In response, one family of large bacteriophages uses a nucleus-like compartment to protect its replicating genomes by excluding host defence factors. Here we find that the bacteriophage nuclear shell assembles primarily from one protein, which we name chimallin (ChmA). Combining cryo-electron tomography of nuclear shells in bacteriophage-infected cells and cryo-electron microscopy of a minimal chimallin compartment in vitro, we show that chimallin self-assembles as a flexible sheet into closed micrometre-scale compartments. We find that the shell is primarily composed of a single protein, chimallin, which self-assembles through its extended N and C termini into a closed compartment.

Size-exclusion chromatography coupled to multi-angle light scattering (SEC–MALS) of purified chimallin indicated a mixture of oligomeric states including monomers, well-defined assemblies of approximately 1.2 MDa, and larger heterogeneous species ranging from 4 to 13 MDa (mean of 6.9 MDa). Cryo-ET of the largest species revealed pleomorphic, closed compartments with near-identical morphology to the phage nuclear shell that we observe in situ. Analysis of the smaller, more defined assemblies by cryo-ET revealed a near-homogeneous population of cubic assemblies with a diameter of around 22 nm, and a minor population of rectangular assemblies with dimensions of approximately 22 × 33.5 nm. Two-dimensional class averages revealed that each cubic particle consists of six chimallin tetramers (24 protomers, 1.67 MDa) arranged to form a minimal closed compartment with apparent octahedral (O, 432) symmetry. Three-dimensional reconstruction of the cubic particles with enforced O symmetry resulted in an approximately 4.4 Å-resolution density map with distorted features, probably arising from the inherent plasticity of these assemblies breaking symmetry. Using the maps for the tetrameric face and full cubic assembly, we built models for the higher-order chimallin oligomers to understand the subunit interconnectivity. CTS1 extends from one protomer to a neighbouring protomer positioned anticlockwise around the three-fold symmetry axis of the cube, and CTS2 further extends anticlockwise to the third subunit around the same axis. Although the linkers between the C-terminal domain and CTS1 (residues 582–589) and between CTS1 and CTS2 (residues 612–621) are unresolved in our maps, we could confidently infer the path of each protomer’s C terminus within the cubic assembly. Compared with the tightly packed chimallin tetramers mediated by the well-ordered NTS region, the length and flexibility of the linkers between the chimallin C-terminal domain, CTS1 and CTS2 suggest that flexible inter-tetramer packing enables chimallin to assemble into structures ranging from a flat sheet to the observed cubic assembly.

>[24x]SNAMIRDTATNTTQTQAAPQQAPAQQFTQAPQEKPMQSTQSQPTPSYAGTGGINSQFTRSGNVQGGDARASEALTVFTRLKEQAVAQQDLADDFSILRFDRDQHQVGWSSLVIAKQISLNGQPVIAVRPLILPNNSIELPKRKTNIVNGMQTDVIESDIDVGTVFSAQYFNRLSTYVQNTLGKPGAKVVLAGPFPIPADLVLKDSELQLRNLLIKSVNACDDILALHSGERPFTIAGLKGQQGETLAAKVDIRTQPLHDTVGNPIRADIVVTTQRVRRNGQQENEFYETDVKLNQVAMFTNLERTPQAQAQTLFPNQQQVATPAPWVASVVITDVRNADGIQANTPEMYWFALSNAFRSTHGHAWARPFLPMTGVAKDMKDIGALGWMSALRNRIDTKAANFDDAQFGQLMLSQVQPNPVFQIDLNRMGETAQMDSLQLDAAGGPNAQKAAATIIRQINNLGGGGFERFFDHTTQPILERTGQVIDLGNWFDGDEKRDRRDLDNLAALNAAEGNENEFWGFYGAQLNPNLHPDLRNRQSRNYDRQYLGSTVTYTGKAERCTYNAKFIEALDRYLAEAGLQITMDNTSVLNSGQRFMGNSVIGNNMVSGQAQVHSAYAGTQGFNTQYQTGPSSFY>METFEISDFKEHAKKKSMWAGALNKVTISGLMGVFTEDEDLMALPIHRDHCPALLKIFDELIVNATDHERACHNKTKKVTYIKISFDKGVFSCENDGPGIPIVKHEQASLIAKRDVYVPEVASCYFLAGTNINKAKDCIKGGTNGVGLKLAMVHSQWAILTTADGSQKYVQHINQRLDNIEPPTITPSREMFTRIELMPVYQELGYAQPLSETEQADLSAWIYLRACQCAAYVGKGTTIYYNDKPCSTSSVMALAKMYTLVTAPNSTIYTATIKADAKPYSLHPLQVAAVVSPKFKKFEHVSIINGVNCVKGEHVTFLKKAINEMVVKKFQQTI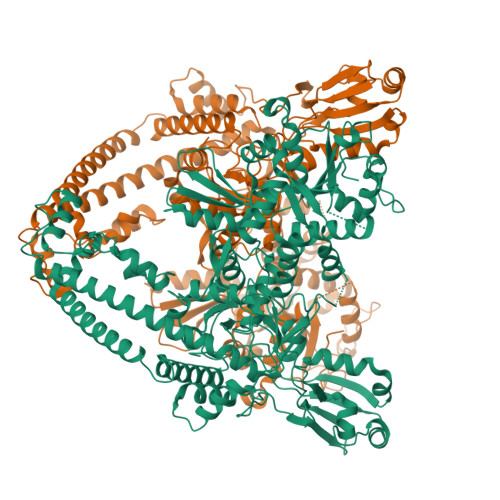KDKNRKTTLRDSCSNIFVVIVGSIPGIEWTGQRKDELSIAENVFKTHYSIPSSFLTSMTRSIVDILLQSISKKDNHKQIDVDKYTRARNAGGKKAQDCMLLAAEGDSALSLLRAGLTLGKSNPSGPSFDFCGMISLGGVIMNACKKVTNITTDSGETIMVRNEQLTNNKVLQGIVQVLGLDFNCHYKTQEERAKLRYGCIVACVDQDLDGCGKILGLLLAYFHLFWPQLIVHGFVKRLLTPLIRVYEKGNTVPVEFYYEQEFDAWAKKQTSLANHTVKYYKGLAAHDTHEVKSMFKHFDKMVYTFTLDDSAKELFHIYFGGESELRKRELCTGVVPLTETQTQSIHSVRRIPCSLHLQVDTKAYKLDAIERQIPNFLDGMTRARRKILAGGLKCFASNNRERKVFQFGGYVADHMFYHHGDMSLNTSIIKAAQYYPGSSHLYPVFIGIGSFGSRHLGGKDAGSPRYISVQLASEFIKTMFPTEDSWLLPYVFEDGQRAEPEYYVPVLPLAIMEYGANPSEGWKYTTWARQLEDILALVRAYVDKNNPKHELLHYAIDHKITVLPLRPSNYNFKGHLKRFGQYYYSYGTYVVSEQRNMITITELPLRVPTVAYIESIKKSSNRMAFIEEIVDYSSSETIEILVKLKPNSLSRIMEEFKETEEQNSIENFLRLRNCLHSHLNFVKPKGGIIEFNSYYEILYAWLPYRRDLYQKRLMRERAVLKLRLIMETAIVRYINESADLNLSHYEDEKEAGRILSEHGFPPLNQSLITSPEFATIEELNQKALQGCYTYILSLQARELLIAAKTRRVEKIKKMQARLDKVEQLLQESPFPGASVWLEEIDAVEKAIIKGRNTQWKFHHH[2x]> 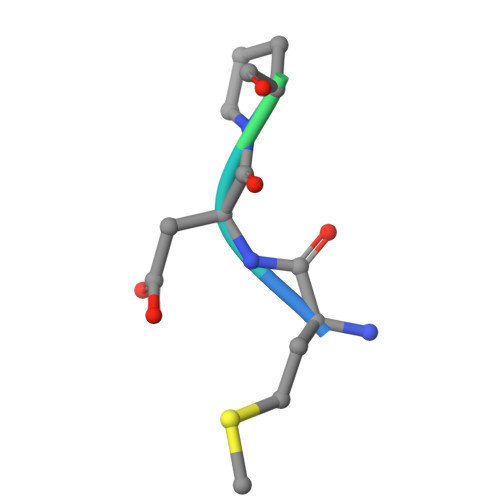MDPVDPNIE>MGAMKNCVIVSAVRTAIGSFNGSLASTSAIDLGATVIKAAIERAKIDSQHVDEVIMGNVLQAGLGQNPARQALLKSGLAETVCGFTVNKVCGSGLKSVALAAQAIQAGQAQSIVAGGMENMSLAPYLLDAKARSGYRLGDGQVYDVILRDGLMCATHGYHMGITAENVAKEYGITREMQDELALHSQRKAAAAIESGAFTAEIVPVNVVTRKKTFVFSQDEFPKANSTAEALGALRPAFDKAGTVTAGNASGINDGAAALVIMEESAALAAGLTPLARIKSYASGGVPPALMGMGPVPATQKALQLAGLQLADIDLIEANEAFAAQFLAVGKNLGFDSEKVNVNGGAIALGHPIGASGARILVTLLHAMQARDKTLGLATLCIGGGQGIAMVIERLNLEHHHHHH[4x]

Here, we present the crystal structure of C. acetobutylicum thiolase (CaTHL), a type II biosynthetic thiolase that catalyses the first step of n-butanol biosynthesis and condenses two acetyl-CoAs to acetoacetyl-CoA. We reveal that CaTHL, unlike other type II biosynthetic thiolases from aerobic bacteria, is regulated via modulation of a redox-switch, indicating that n-butanol production and the relevant metabolic fluxes in Clostridium are tightly regulated by thiolase. CaTHL consists of three domains: an N-terminal α/β domain (N-domain, residues 1–119 and 249–269), a loop domain (L-domain, residues 120–248), and a C-terminal α/β domain (C-domain, residues 270–392). The N- and C-domains form a typical five-layered fold (α–β–α–β–α) observed in other thiolase superfamily of proteins including peroxisomal degradative thiolase from Saccharomyces cerevisiae, β-ketoacyl synthase II from E. coli, and the biosynthetic thiolase from Zoogloea ramigera (ZrTHL)14151617181920.

For comparison, the crystal structure of EcTHL was also determined at 2.10 Å resolution. As hypothesized, there was no disulfide bond formation observed between the two catalytic cysteine residues, Cys89 and Cys379, under oxidized condition. In addition to the absence of a disulfide bond, the catalytic cysteine loop and the flexible region had similar conformations to those of the reduced form of CaTHL, confirming that EcTHL is also non-redox-switch regulated. The flexible regions of EcTHL and ZrTHL are well stabilized by direct and water-mediated hydrogen bond network; on the other hand, in CaTHL, strong hydrogen bond interactions are not observed between the flexible region and its surrounding region. Considering that the flexible region of CaTHL undergoes an order-to-disorder conformational change depending on the disulfide bond formation, it seems that the stability of the flexible region of CaTHL is not sufficiently high, leading to disulfide bond formation under oxidized condition. This would confer the redox-switch regulatory mechanism to the enzyme; on the other hand, the highly stabilized flexible regions of EcTHL and ZrTHL disable the rotation of the Cys378 residue and hence prevent disulfide bond formation. On the other hand, ZrTHL and EcTHL seem to be permanently inactivated upon the oxidation of the corresponding catalytic cysteine residues to sulfinic or sulfonic acid, and cannot be switched back to the active enzymes under reducing condition.>MS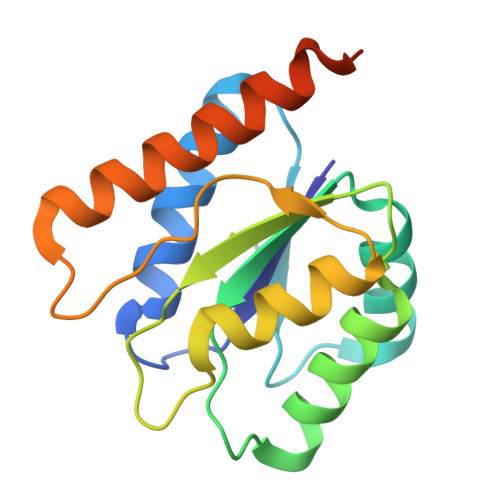VLIGYLSDYGYSDRLSQAIGRGLVKTGVAVEMVDLRAVDPQELIEAVSSARGIVLGTPPSQPSEAVATALSTIFAAAHNKQAIGLFDSYGGDDEPIDALLAQFRNLGLHTAFPPIRVKDQPTEAIYQQCEESGTDLGQWLTRADAIQTMKSLEHHHHHH[3x]>[2x]SNGLEDSSTISFITWNIDGLDGCNLPERARGVCSCLALYSPDVVFLQEVIPPYCAYLKKRAASYTIITGNEEGYFTAILLKKGRVKFKSQEIIPFPNTKMMRNLLCVNVSLGGNEFCLMTSHLESTR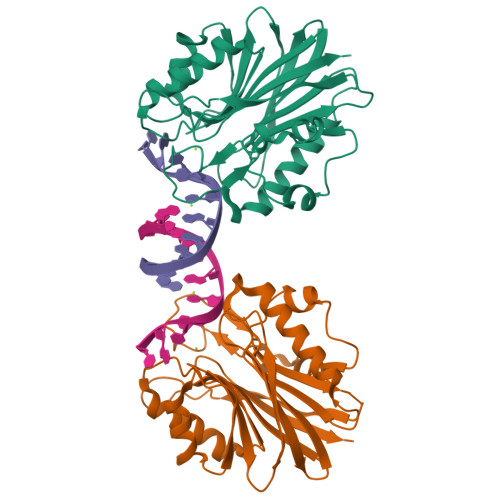EHSAERIRQLKTVLGKMQEAPDSTTVIFAGDTNLRDQEVIKCGGLPDNVFDAWEFLGKPKHCQYTWDTKANNNLRIPAAYKHRFDRIFFRAEEGHLIPQSLDLVGLEKLDCGRFPSDHWGLLCTLNVV>MSEITGLFKDLTKVKHARNGRLASWDQRGKNQDYWEIPAGESITLGEIEGPGCITHMWMTSSCRKVVAPSILDPELNASAAPVMEIHPALGVIWDAYDPFYYRKALIKITWDDQDTPSVLVPFGDFFCIGNSYPGNFSSLPFNVSLKPEEAGKFGAPCSVSCYFPMPFNKKAKIEIVNDNELPFILYFNIDYEMYGEPLPEDTAYFHAAWHRENPCNGWGPELQVNSPEVNNVTNFKGENNYTVLDVEGTGHYVGCNLTVKHFQGSWWGEGNDMFFIDGEEYPSLNGTGTEDYFNHAWGMQRNAYPFFGTIVHEGDTDGFQVSYRWH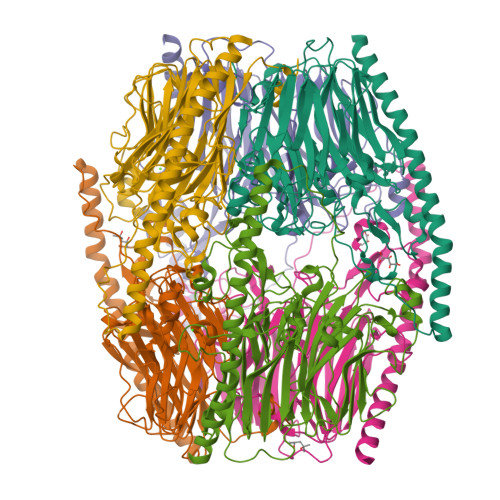ITDPVRFEKHLKVTIEHGHANQLSDDWSSTAYWYQILPTASRITIAPVEDRLPVVPQLPERKLVLPQLTEEQQAARDTYQKRWKDYEPRRDTQFRIKEDKARRESKLNTEFAKKLRDAFDAEREQLEHHHHHH[6x]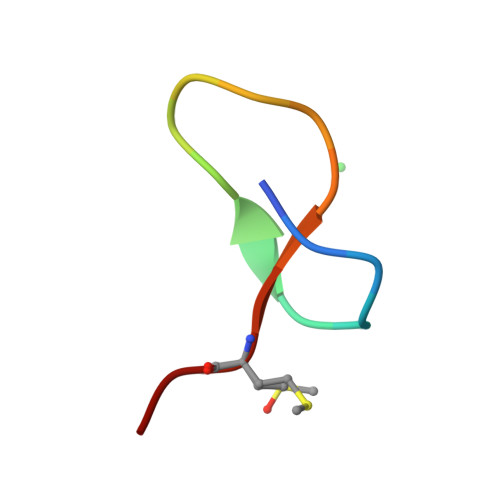> GTLTPGLPEDFLPGHYMPG>[2x]MRARLYAAFRQVGEDLFAQGLISATAGNFSVRTKGGFLITKSGVQKARLTPEDLLEVPLEGPIPEGASVESVVHRE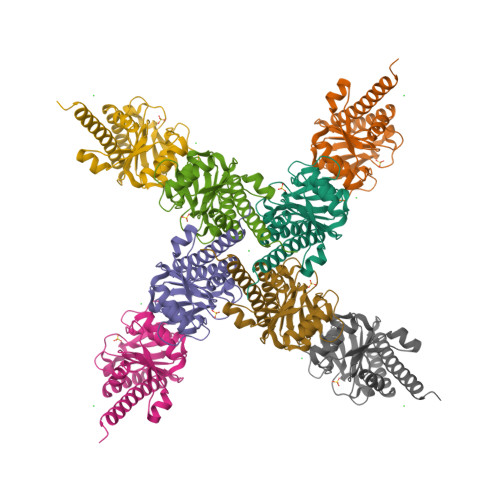VYRRTGARALVHAHPRVAVALSFHLSRLRPLDLEGQHYLKEVPVLAPKTVSATEEAALSVAEALREHRACLLRGHGAFAVGLKEAPEEALLEAYGLMTTLEESAQILLYHRLWQGAGPALGGGE> MVCTFFENKVCVETMEDHIRK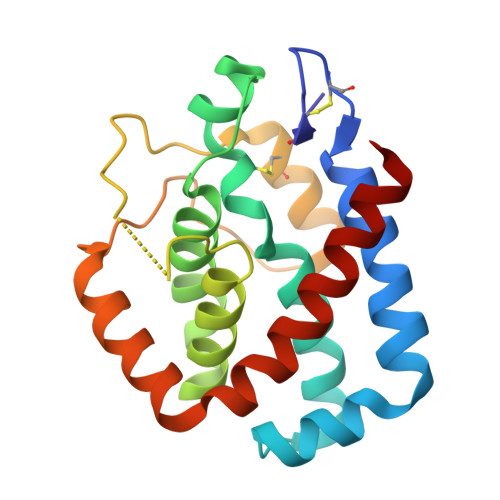GLEIIEGLYLRRGYGHFLSKILNIDVKLAEELLKKAYIFHDIGKCLEEFQQRREKFRFHEVYSALVAREVFKKYGDIGGVVSVAILLHHHNWIREKSPKRPRNLKLCNECLSIIKKLSGEKIPEEIPWRNWIEFTEEAEEIMRTNLRGVYSILLPLVVADNYAAAVNR> ANKPMQ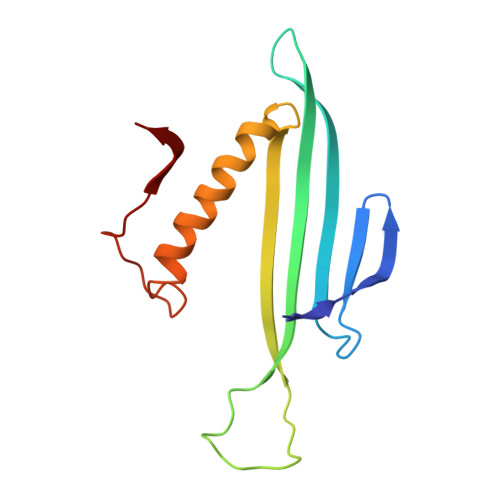PITSTANKIVWSDPTRLSTTFSASLLRQRVKVGIAELNNVSGQYVSVYKRPAPKPEGCADACVIMPNENQSIRTVISGSAENLATLKAEWETHKRNVDTLFASGNAGLGFLDPTAAIVSSDTT> MMRCCCVLQDKSMFAAKRRVIVPIHPTPNYPAHFIKASFTTDPLKEKQKARFSSGGEAMREVQMIPKNLEGERSRRELMSRGDTEFEALVEFIQGASYDQLISGRRFKKVYDKLSENDDTFVWLCHTAMSVLNPGDVRSRLVYNHLRTLAEAVANGEMTLRTAFRFYESAVRSPAYREIAKRQMEGGAATRLAGISAAADVMRRMGLTRRPMASYFELYQRIVERSEAMTPWGFPPLFQFEERLSLEPRLKFFSRA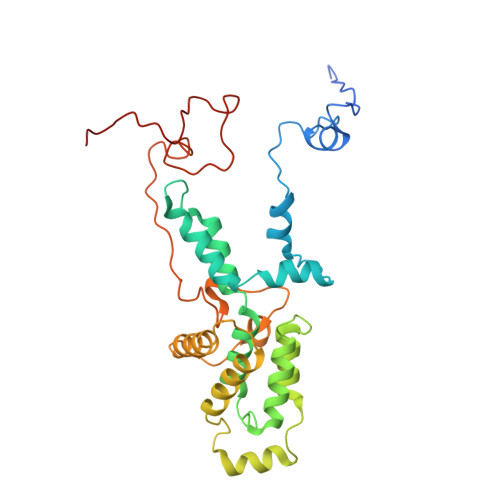SQQALERRRRGHIMSAYTTLQGRRIFWIPPTWNRAGRFLGPHVTLYPGMTPD> SELDAKLNKLGVDRIAISPYKQW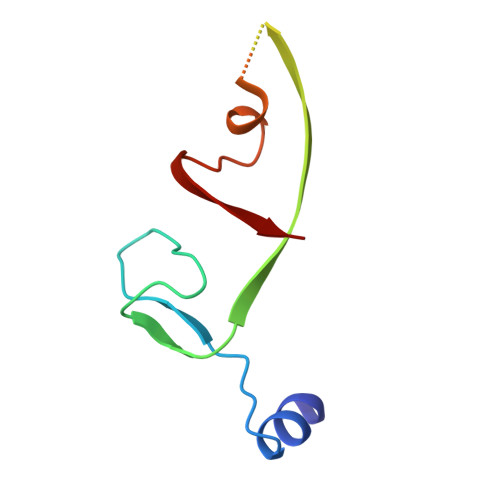TRGYMEPGNIGNGYVTGLKVDAGVRDKSDDDVLDGIVSYDRAETKNAYIGQINMTTAS We show that indeed Sfm1 consists of a typical SPOUT domain at the N-terminus flanked by a small C-terminal domain (CTD). Sfm1 exists as a monomer and exhibits a negatively charged surface surrounding the active site unsuitable for RNA binding. Consistently, Sfm1 has no activity towards RNAs but can specifically catalyze the Arg146 methylation of yeast and human S3, and the CTD is critical to the substrate binding and the activity. Sfm1 is the first SPOUT protein that can catalyze protein arginine methylation.

The crystal structure of a C-terminal truncated Sfm1 (Sfm1ΔC: residues 1−204) in apo form was solved by the single-wavelength anomalous dispersion method at 2.0 Å resolution and refined at 1.9 Å resolution, and the crystal structure of the full-length Sfm1 (residues 1−213) in complex with S-adenosyl-homocysteine (SAH) was determined by the molecular replacement method at 2.5 Å resolution. In the SAH-bound Sfm1 structure, both molecules are well defined except for residues 1 and 205−213 of molecule A and residues 1, 172−175 and 205−213 of molecule B, and the C-terminal his-tag and the linker are disordered in both molecules. In the SAH-bound Sfm1 structure, SAH is clearly defined in the electron density map. SAH binds to a pocket formed by the three connecting loops of the trefoil knot (residues 83−92, 105−115 and 131−140, referred as L1, L2 and L3 loops, respectively), and assumes a bent conformation, similar to that in the structures of other SPOUT MTases. The adenine moiety of SAH has largely hydrophobic interactions with Pro85 of the L1 loop and Leu133 and Met138 of the L3 loop, and additionally the N6 group of the adenine moiety forms three hydrogen bonds with the main-chain carbonyl groups of Leu133, Gly134 and Lys136 of the L3 loop. The 2'-OH and 3'-OH groups of the ribose moiety form a hydrogen bond with the main-chain carbonyl group of Leu83 of the L1 loop and the main-chain amine group of Gly105 of the L2 loop, respectively. The homocysteine moiety interacts with the main-chain amine and carbonyl groups of Ile107 of the L2 loop via its carboxyl group and interacts with the main-chain carbonyl group of Met8 of the β1-α1 loop and a water molecule via its amine group. In the SAH-bound Sfm1 structure, the two molecules in the ASU are related by a pseudo two-fold symmetry (about 180°) and the intermolecular interface involves mainly α1, α6 and η1 (or the equivalent loop) of the SPOUT domain in both molecules. Structural comparison shows that the apo and the SAH-bound Sfm1 assume very similar overall structure (root-mean-square deviation of 1.2 Å for 202 Cα atoms); however, the SAH binding induces some notable conformational changes at the active site. Particularly, on the cofactor binding, the β5-α5 or L2 loop, the following α5 helix, and the β1-α1 loop move towards SAH by about 3.0 Å.

>MKYIIEHMEEGFSEWVILEYSQILREVGAENLILSSLPESTTEKDIPQRLLKLGLRWTTKDLKGINEDFKDLELLKDGRVCLLDPRATIDLQPEDATKFDYFVFGGILGDHPPRDRTKELKTAYPNLLISRRLGDKQMTTDTAIRTTQLIIKDRIAFEDIKFIDYPEFRFNKNEATEMPFRYVLDKEGKPILPEGMLDLIKKDSAQSLDDLLMLEHHHHHH[2x]Mesaconyl Coenzme A | C26 H40 N7 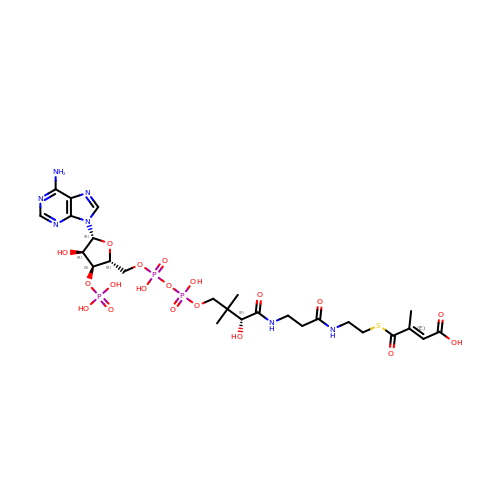O19 P3 S | LVBVWNJPMXCQJE-CBBDEUQJSA-N> YAFNQYLPFPDGMSPFQAAMQDESGYQVHRTLQYEDGAFVTANLRYTYEGSHIKGEFQVIGTGFPPDGPVMTNKLTALDWSVVKFVYPNDKTILSTFDKTYTTTDGKRYQCTFRENNTFAKPMAADILQKQPMFIFHKTELQHSNNAELTFKEKQTAFSDMKSGG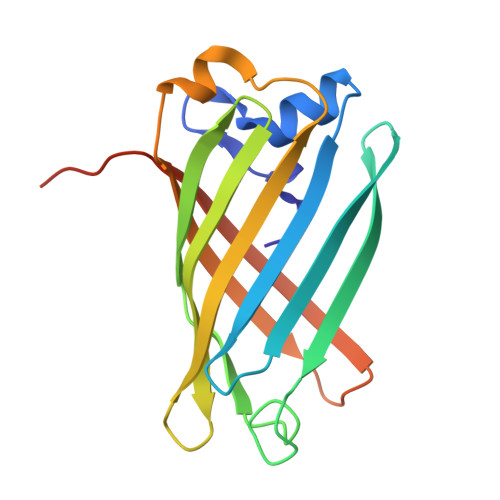SHHHHHH>GPHMLEVPPQPQYSYHDINVYSLAGLAPHITLNPTIPLFQAHPQLKQCVRQAIERAVQELVHPVVDRSIKIAMTTCEQIVRKDFALDSEESRMRIAAHHMMRNLTAGMAMITCREPLLMSISTNLKNSFASALRTASPQQREMMDQAAAQLAQDNCELACCFIQKTAVEKAGPEMDKRLATEFELRKHARQEGRRYCDPVVLTYQAERMPEQIRLKVGGVDPKQLAVYEEFARNVPGFLPTNDL[2x];>[2x]GPHMLEREKIYQWINELSSPETRENALLELSKKRESVPDLAPMLWHSFGTIAALLQEIVNIYPSINPPTLTAHQSNRVCNALALLQCVASHPETRSAFLAAHIPLFLYPFLHTVSKTRPFEYLRLTSLGVIGALVKTDEQEVINFLLTTEIIPLCLRIMESGSELSKTVATFILQKILLDDTGLAYICQTYERFSHVAMILGKMVLQLSKEPSARLLKHVVRCYLRLSDNPRAREALRQCLPDQLKDTTFAQVLKDDTTTKRWLAQLVKNLQE;>[2x]X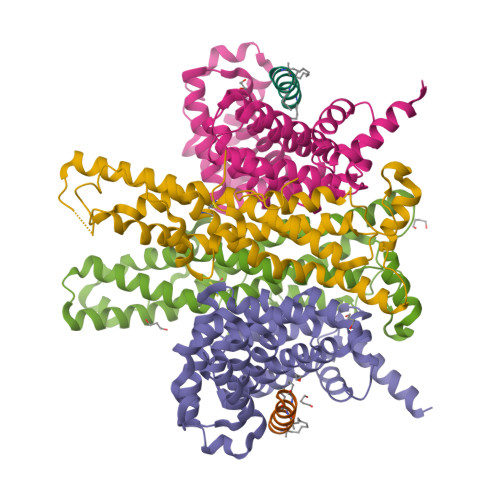LDLNFKLLEEHLALLVEX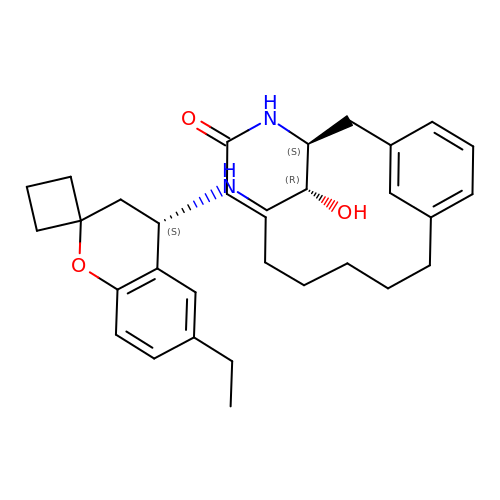(3S)-3-[(1R)-2-{[(4S)-6-ethyl-3,4-dihydrospiro[chromene-2,1'-cyclobutan]-4-yl]amino}-1-hydroxyethyl]-4-azabicyclo[11.3.1]heptadeca-1(17),13,15-trien-5-one | C32 H44 N2 O3 | QPAQZVPVDCXNCF-YTCPBCGMSA-N> SYSPEPDQRRTLPPGWVSLGRADPEEELSLTFALRQQNVERLSELVQAV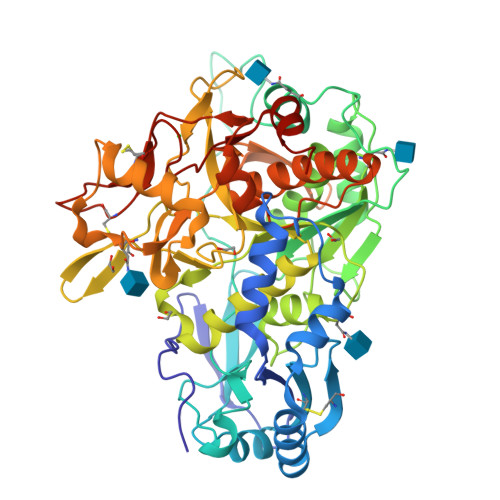SDPSSPQYGKYLTLENVADLVRPSPLTLHTVQKWLLAAGAQKCHSVITQDFLTCWLSIRQAELLLPGAEFHHYVGGPTETHVVRSPHPYQLPQALAPHVDFVGGLHRFPPTSSLRQRPEPQVTGTVGLHLGVTPSVIRKRYNLTSQDVGSGTSNNSQACAQFLEQYFHDSDLAQFMRLFGGNFAHQASVARVVGQQGRGRAGIEASLDVQYLMSAGANISTWVYSSPGRHEGQEPFLQWLMLLSNESALPHVHTVSYGDDEDSLSSAYIQRVNTELMKAAARGLTLLFASGDSGAGCWSVSGRHQFRPTFPASSPYVTTVGGTSFQEPFLITNEIVDYISGGGFSNVFPRPSYQEEAVTKFLSSSPHLPPSSYFNASGRAYPDVAALSDGYWVVSNRVPIPWVSGTSASTPVFGGILSLINEHRILSGRPPLGFLNPRLYQQHGAGLFDVTRGCHESCLDEEVEGQGFCSGPGWDPVTGWGTPNFPALLKTLLNP>PMVTAATSLRRALENPDSFIVAPGVYDGLSARVALSAGFDALYMTGAGTAASVHGQADLGICTLNDMRANAEMISNISPSTPVIADADTGYGGPIMVARTTEQYSRSGVAAFHIEDQVQTKRCGHLAGKILVDTDTYVTRIRAAVQARQRIGSDIVVIARTDSLQTHG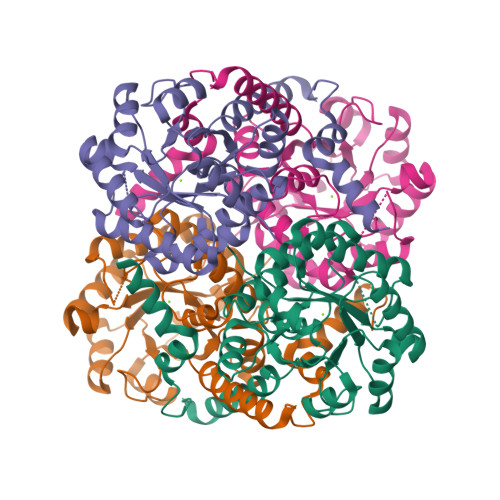YEESVARLRAARDAGADVGFLEGITSREMARQVIQDLAGWPLLLNMVEHGATPSISAAEAKEMGFRIIIFPFAALGPAVAAMREAMEKLKRDGIPGLDKEMTPQMLFRVCGLDESMKVDAQAGGAAFDGGVDLK[12x]>[2x]SNAVTATQLAAK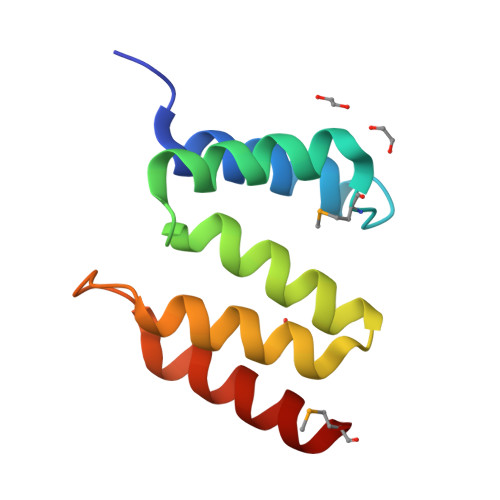ATTLYYLHKQAMTDEVSLLLEQALQLEPYNEAALSLIANDHFISFRFQEAIDTWVLLLDSNDPNLDRVTIIESINKAKKLM> GSSHHHHHHSGDPASMNNHPEVKIKTILSLFLNINIDDFNMDANLADAYDMDSTELADLAKEIEKEFGISVTKSQFSHWETGRAVLDFVSSSLNDKN;>[3x]GSSHHHHHHSGDPASMIINNRNESQPRRVVVTGLGVVAPTGVGVNEFWNNIHNGKSGVSKYEWGRERFGFKSGAIGQVYGSDGNNKEFVLKSERKYLQFALDAAEMAMQDANLRPSDIDGRRFGVAIATAIADAAGMEECLLRITKGGKENIHPDLIKSEDYDSFDFSSAATSVAKKYGASMSVSNISTGCAAGLDALGIAME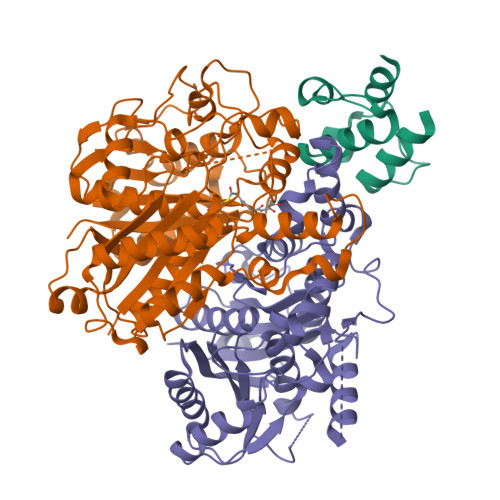HIRYGRADIMLAGASEAPLCPLSIGSFEALGALSSRELENQQAATCPFSLERDGFVIAEGCGILILESYEHAKQRGAHIYAELAGYASVNNAYHMTDLPADGMAMARCIDMALKDAQISPSTVNYISAHGSSTAQNDINESNAIKFVLGESAFGIPINSLKSMTGHALAAANAIESVALCLEIEKQYVHPTINYQTPDPDCDLDYIPNQGCSYPIKTALKLSSGFSGIHSVIVMRAVDNA;>[3x]MRKRVVVTGVGAIHPDGNDVTAIKSKVIQKLLGQESKNNTTASSIIRTLSDFDGAKYINNRLRRKIDEFSVYGIVAVEMALKASRLDVDKLDPNRVGIYVGNCFGGWQHIEDEVKALHIEGIKGMGPYVATAWFPAALQGQLSLLYGFSAQSKTFSTSDVAGMQAIGYAAEAISNGVAEVMLCGASEHLSSPLVKNLLEKTSSQKHSEVFGEKQPGDFSEGAAFLVLEERQHALERGASILCELTGFVDYFAPDKNTRNNTLEYTAELFNHNENAVFIMDGIYDDEKEITSKAFSNKEIKTSFINLRPYLDNQFSVSGVIDSVLASSFLSESHGDEEQQSKKINEFSNTNQIIIQRFSNQGHVCALSFSAI2-azanyl-N-[[4-bromanyl-3-(3-chloranyl-5-cyano-phenoxy)-2-fluoranyl-phenyl]methyl]-4-chloranyl-1H-imidazole-5-carboxamide | C18 H11 Br Cl2 F N5 O2 | 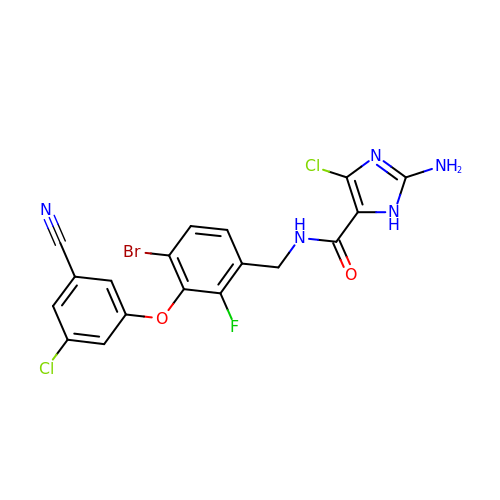IZRLYEGHBQTAFO-UHFFFAOYSA-N Nef from human immunodeficiency virus (HIV) or simian immunodeficiency virus (SIV) is a 27–35 kDa viral accessory protein that is dispensable for replication but required for high infectivity and virulence. Notable among Nef’s functions is the interaction of Nef with TCRζ, the principal signaling component of the T-cell antigen receptor. In previous work, SIV and HIV-2 Nef have been shown to bind TCRζ at two unique sites denoted ‘SIV Nef interaction domains’ (SNIDs), the first containing elements of immunoreceptor tyrosine activation motif (ITAM) 1 and the second containing elements of ITAM 2. The Nef conserved core domain (Nefcore) has been described to be responsible for the majority of Nef’s interactions, including the TCRζ-binding activity of SIV Nef.

In the presence of the shorter 18-residue TCRζA63–R80 polypeptide the complex unexpectedly crystallized in the P212121 space group with severe pseudo-hemihedral twinning. Ultimately, a partially twinned crystal with a twin fraction of 0.426 was used to solve the structure of the SIVmac239 Nefcore–TCRζA63–R80 complex to 2.05 Å resolution. M was calculated to be 2.64 Å3 Da−1 (53.42% solvent) for crystal 1 and 2.64 Å3 Da−1 (53.99% solvent) for crystal 2, which is consistent with two SIVmac239 Nefcore–TCRζA63–R80 heterodimers comprising the asymmetric unit. Two nearby molecules (A and  B) in the same twin domain related by an approximate 90° rotation were selected to comprise the asymmetric unit. Clear density for the TCRζA63–R80 polypeptide ligand was observed and this region was also built into the structure, with 13 of the 16 resolved residues comprising a canonical α-helix. The P212121 crystal form contained two molecules per asymmetric unit which were no longer related by a crystallo­graphic twofold symmetry operation (y, x, −z) but instead by a twofold NCS operation, In the tetragonal crystal form the SIVmac239 Nefcore–TCRζDP1 complex and its symmetry-related partner (y, x, −z) form an antiparallel dimer similar to the crystallographic dimer described previously for the HIV-1 Nefcore. Structural alignment of one SIVmac239 Nefcore–TCRζA63–R80 complex from the P212121 crystal form with its corresponding molecule in the P43212 crystallographic dimer reveals that the NCS-related molecule in the orthorhombic crystal form is rotated by ∼10° from its corresponding molecule in the P43212 crystal form. TCRζ residue Gln65 additionally participates in hydrogen bonding to the main-chain amide and carbonyl of residues Arg103 and Val102, respectively, on its bound SIVmac239 Nefcore partner. Interestingly, this inter­action orders the proline-rich region in the N-terminus of the bound SIVmac239 Nefcore into a polyproline type II (PPII) helix as evidenced by the clearly resolved electron-density maps calculated from the P212121 crystal data for that region.

>[2x]GSDDLVGVSVRPKVPLRTMSYKLAIDMSHFIKEKGGLEGIYYSARRHRILDIYLEKEEGIIPDWQDYTSGPGIRYPKTFGWLWKLVPVNVSDEAQEDEEHYLMHPAQTSQWDDPWGEVLAWKFDPTLAYTYEAYVRYPEEFGS;>AYQQGQNQLYNELNLGRR[2x]> GGWVSGE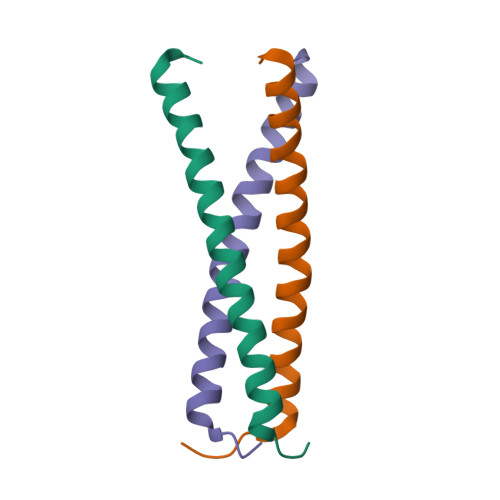EFYMLTRRVLQLETVLEGVVSQIDAVGSKLKMLERKGW S-5'-AZAMETHIONINE-5'-DEOXYADENOSINE | 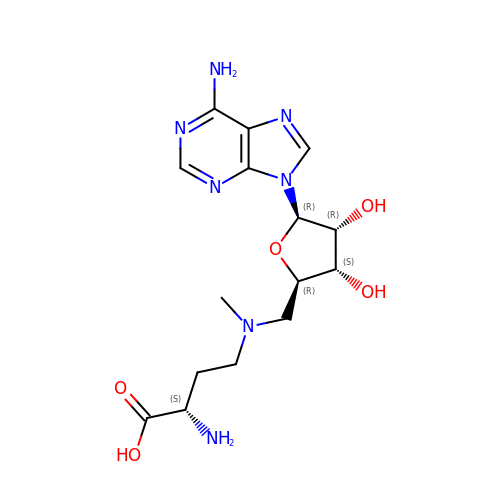C15 H23 N7 O5 | JISVTSUBJCPLSV-TWBCTODHSA-N At present, the best structurally characterized pLGIC is the G. violaceus ligand-gated ion channel (GLIC), of prokaryotic origin. Each subunit consists of an extracellular domain (ECD), predominantly in a β-sandwich fold, and a transmembrane domain (TMD) composed of four helices, labeled M1–M4. However, the GLIC is a pH-gated channel, activated by lowering the pH, with a maximal activation at pH 4 and a pH50 around 5. We instead found that proton activation is a complex multiple loci mechanism, with the key contribution stemming from the coupling interface between the extracellular and transmembrane domain, with E35 acting as a key proton-sensing residue.

In the lower part of the ECD, the principal (+) face also carries two acidic residues, E82 and D115. E82Q and D115N display significantly higher proton sensitivity than E82A and D115A, respectively. Assuming that Gln and Asn faithfully mimic protonated side chains of Glu and Asp, this would suggest that residues E82 and D115 are also proton sensors. To investigate this idea, the structures of E82Q and E82A were solved at pH 4. The E82A structure is similar to that of the Wt pH 4 structure, whereas that of E82Q shows a marked local reorganization of the Q82 moiety. A structural analysis was performed on E26Q, E26A, E35Q, E35A, E67A, E75A, E82Q, E82A, D86A, D88N, D88A, H127N, E181A, and H277Q mutants, by solving their structure at pH 4. All structures were in the apparently open conformation.

>[5x]GQDMVSPPPPIADEPLTVNTGIYLIECYSLDDKAETFKVNAFLSLSWKDRRLAFDPVRSGVRVKTYEPEAIWIPEIRFVNVANARDADVVDISVSPDGTVQYLERFSARVLSPLDFRRYPFDSQTLHIYLIVRSVDTRNIVLAVDLEKVGKNDDVFLTGWDIESFTAVVKPANFALEDRLESKLDYQLRISRQYFSYIPNIILPMLFILFISWTAFWSTSYEANVTLVVSTLIAHIAFNILVETNLPKTPYMTYTGAIIFMIYLFYFVAVIEVTVQHYLKVESQPARAASITRASRIAFPVVFLLANIILAFLFFGF> GPLGSPEFPGRRKPEAQPFAHLTINAASIPSGSHKVTLSSWYHDRGWAKISNMTLSNGKLRVNQDGFYYLYANICFRHHETSGSVPTDYLQLMVYVVKTSIKIPSSHNLMKGGSTKNWSGNSEFHFYSINVGGFFKLRAGEEISIQVSNPSLLDPDQDATYFGAFKVQDID;> VTPPCTQERHYEHLGRCCSRCEPGKYLSSKCTPTSDSVCLPCGPDEYLDTWNEEDKCLLHKVCDAGKALVAVDPGNHTAPRRCACTAGYHWNSDCECCRRNTECAPGFGAQHPLQLNKDTVCTPCLLGFFSDVFSSTDKCKPWTNCTL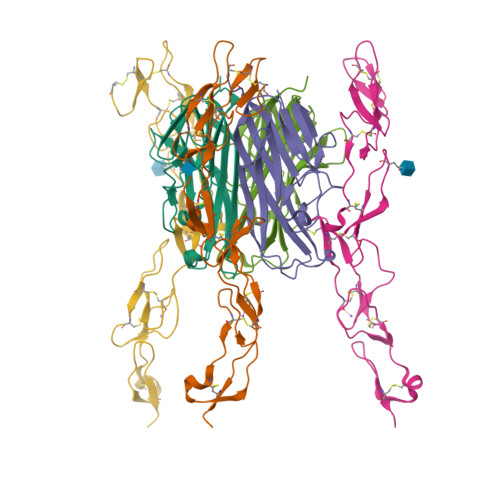LGKLEAHQGTTESDVVCSSSGSLVPR4-[4-[2-(5-bromanyl-1~{H}-indol-3-yl)ethyl]pyrimidin-2-yl]morpholine | C18 H19 Br N4 O | 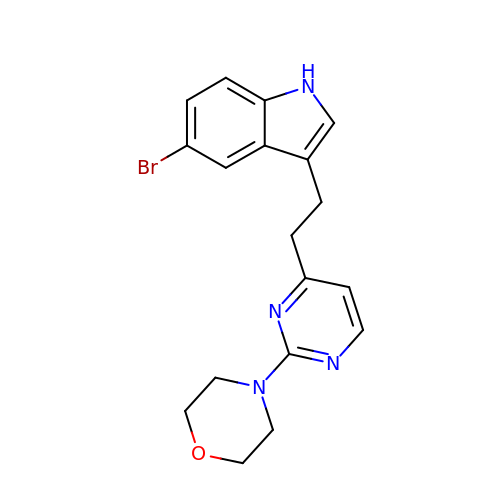LPEIQZYVQYBIQO-UHFFFAOYSA-N>MTIDINKLKEELGLGDLAKSLEGLTAAQKAQEAERMRKEQEEKELARMNALVSKAVGEDRQKLEQALELVKSLDEKSKKSAELFAQTVEKQQETIVGLQDEIKSLLTAREGRSFVGDSVAKALYGTQETFEDEVEKLVLLSYVMEKGVFETEHGQKHLKAVNQSSSVEVSSESYETIFSQRIIRDLQKELVVGALFEELPMSSKILTMLVEPDAGRATWVAASAYGSDNTTGSEVTGALTEIHFSTYKLAAKSFITDETEEDAIFSLLPLLRKRLIEAHAVSIEEAFMTGDGSGKPKGLLTLASEDSAKVTTEAKADGSVLVTAKTISKLRRKLGRHGLKLSKLVLIVSMDAYYDLLEDEEWQDVAQVGNDAVKLQGQVGRIYGLPVVVSEYFPAKAAGKEFAVIVYKDNFVMPRQRAVTVERERQAGKQRDAYYVTQRVNLQRYFENGVVSGAYAAS[13x]

The T5 family of viruses are tailed bacteriophages characterized by a long non-contractile tail. The bacteriophage DT57C is closely related to the paradigmal T5 phage, though it recognizes a different receptor (BtuB) and features highly divergent lateral tail fibers (LTF). We present a composite map determined by electron cryo-microscopy (cryo-EM) at resolutions ranging between 2.9 Å to 4.9 Å of the entire T5-like phage particle DT57C, and atomic models comprising its core structural proteins. Our results provide a complete atomic structure of a T5-like phage, provide insights into the process of DNA ejection as well as a structural basis for the design of engineered phages and future mechanistic studies.

Furthermore, we could separate the particle population into pre-ejection (capsid filled with DNA) and post-ejection (empty capsid after DNA release) states and to reconstruct the related states of the portal complex and the tail tip individually at resolutions sufficient to build atomic models of each state, gaining insight into the conformational changes leading to DNA release. Using 2D classification, we identified a smaller population of phages (~20% of all particles), where their DNA had been ejected. Following a similar methodology as for the intact phages (representing the pre-ejection state), we obtained reconstructions of the different parts of these empty phages (corresponding to the post-ejection state). Consistent with structures of the closely related T5 phage, the T = 13 icosahedral capsid of mature DT57C was composed of two proteins, the major capsid protein (MCP) and the head decorating protein (DCP), and it had a diameter of 930 nm. The asymmetric unit comprises 13 copies of the MCP lacking the Δ-domain (the first 160 N-terminal residues, which is cleaved during the maturation process of the capsid). To further confirm that empty phages indeed correspond to a post-ejection state where both the DNA and the bulk of the TMP had been properly ejected through the tail, we compared tomograms of virions in three different states: empty virions with an intact capsid, filled virions with an intact capsid and empty virions with a broken capsid. The tomograms revealed that nearly all empty virions have an intact capsid.>[10x]MATSASSHLNKGIKQVYMALPQGDKVQAMYIWIDGTGEGLRCKTRTLDSEPKCIEELPEWNFDGSSTFQSEGSNSDMYLVPAAMFRDPFRKDPNKLVFCEVFKYNRKPAETNLRHTCKRIMDMVSNQRPWFGMEQEYTLMGTDGHPFGWPSNGFPGPQGPYYCGVGADKAYGRDIVEAHYRACLYAGIKIG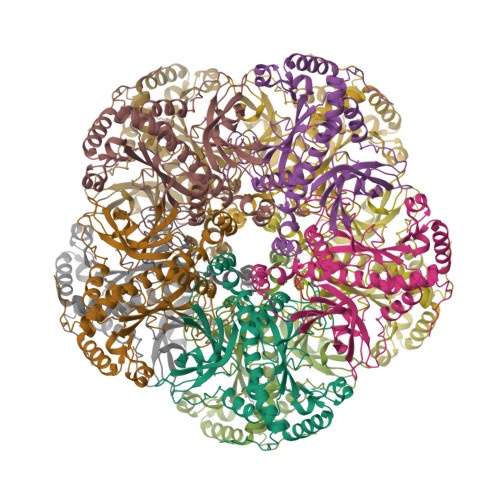GTNAEVMPAQWEFQIGPCEGIDMGDHLWVARFILHRVCEDFGVIATFDPKPIPGNWNGAGCHTNFSTKAMREENGLKYIEEAIEKLSKRHQYHIRAYDPKGGLDNARRLTGFHETSNINDFSAGVANRGASIRIPRTVGQEKKGYFEDRRPSANCDPFAVTEALIRTCLLNETGDEPFQYKN5-(1-methylpyrazol-4-yl)-3-(3-phenoxyphenyl)furo[3,2-b]pyridine | 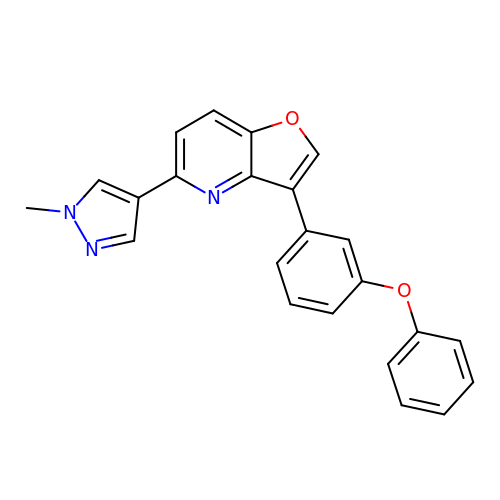C23 H17 N3 O2 | RDHFKBABHOAOCH-UHFFFAOYSA-N(3S)-1,2,4-triazolidin-3-amine | C2 H8 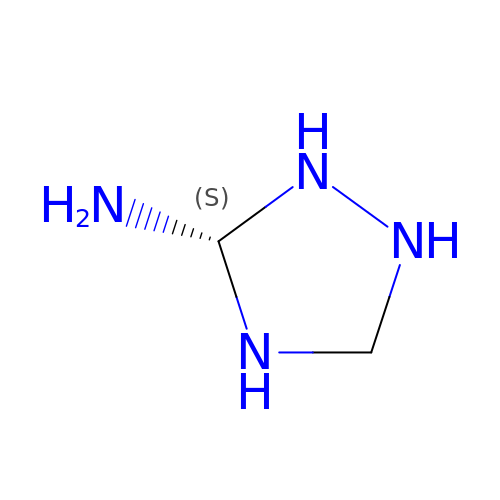N4 | OKGXDOJTXCDXPH-UWTATZPHSA-N> MSNLFRSLASSMRALSLAAPRATAVNTTKTVVSTHQTRCLSQGLLSRHICTPMCSHNRPVAVCQSAKNGLQSKQQSRGMKVHSAIKKRCEHCKVVRRKANKRQNGYLYIICPANPRHKQRQGYR;> MSTCQQVARPLVRCLRQTGPGAATCSTRSVAVAAVRPFSSTPMRKEEGATTTTTTSPVDSTTTPPPLPSATEAKATVADTVVGGPELGSRRRRAALATTGNLPFEQLPYQCFQDARKILQQDRAAKIAQIVKETEKIKLIEARDASEFEGGEAAKQTRIKSLRKYIEELKILADINDPEVKRRFEDGRGDMTKPVYRFMAERRWRSMDYKIIAQRISQFHVVPDLLPAFDPTMDVKLSFRGYQVSPGAILDSRVTEVAPTLRMQVFDKGERLLTVVVIDSDVPDVTHDNFKRRCHFLAANIPWDPSKTVLSLRSVGDRVEGDVGKPWLPPFAQKGSPYHRLNVFVLEQKPGAKIDGEALKKHLENRENFSLKGFREKFDLEPVGFNLFRSEWDEGTAEVMERHGIPGAEVEFKRQKFASLKPPRKARGWEAKRQKPKYKSLWKYVKRIA;> MVSATKKPVSAMSAKNSTRHRKVSHKVTKTIATAKSQVISNKAMKIRTKSWKDMPSPKRRRRINAMVDELRLQGNVKMPKPGKSTYKAGGGERVRLVKAASTLPTPPLTPPVLSKPTGSASQSKGDLKPKRPTPEKKRSVSKRDVERFFLSTQTSTRRRENTPIHAPIMSSTFTSLRGLATRLFAGGARPSPSSLLLPNKPATAALPTAIQHQQTASYASKGKSGPPAGMFSGQKAGSKKSKGPKQVDPRIINILRHFAVLSPKRIPPPLRFGRNRYLRHWTIHRAWLLFRRQQREQRERILMQQHQSMSNACEELRNTEGPGTRETGYLYRVAMLKNGVYGLKSIPIEYASRALVETPGRQAWNHEWKR;> MQPTRILQGLKYRKLRLTTKDVNKGFYKGNRTGSMGTHTSYGTYKIDYTKVRTYVCPDLTGFKLTPFVSKTIRPVHDQFPGDKLGPKNPATYLARWKSENGLD;> MTVKALTQISSAGRNGVGAFVLQCKKLDIHYSDWAGSSRGMNGFIKSLLPKFAAANPQIEFVVSPRPAKHPILMGHYINGRTKAICVRNMEPLEILKKAELLRDASGEKPQKFKKPVTSTNPSVRGVWSPYHGQGMAV;> MKRIATPSLTSRLLVAARSGVSPATAAIRSRSAISVRSQSTAALAQHDASHDLNNDRFPPLEPLPPAAESLPSPLPERALTSAKLAALHARLNLSPKIPLQTLARTLVDASADENPQFNNANLAFVGQTLINYHIAEWLLCKYPRLPQGILFSAMKAYAGPKPLLQIARSWGVDTAAVPGGEVDPGLLQFDALKPGVAITNFGYKRTELAYLEKFKWRRGMASRVVLDDDFGDVVRSDPKVAADLEKAMEEQDQDKTPDEEEAEMVANEQDQDVSYDRYGNPDTRAAAERAHAYFVRAVVGAIYAHCGREAAKAFVKAHIMSRTLDIAKLFEFKYPTRELAALCAREDFEPPVARLLSETGRQSRTPVFVVGIYSGSDKLGEGAASSLDHARFKAAMNALKAWYLYSPGENPRVPSDMLEEGAKPWTPAYIDMGEVISR;> MSASSRGAALLRSQQRSICLQCRNQTRVLAPAGVTSAPRRFYSAEASATATATATATTTTTLPPPHPPVTTSTGTHAATSTSSQIYRIKSGVILTRPPLLTRDLTPFEESFYFYQKRLNERLTAPFRKDFYFKKDTAADLDWRIKLKERHGVPAKDIGRYNPRGRMAWNDEVLVGSQTSSRKHMVEKLLADAEMRVSEDGEEIPAEDRVPVEKPMPRRTEADEKGDVKRLDRALDKTLYLVVKKKADKEGEEAKWMFPTGVVPTDEGLHETAARILAESAGVNMNTWIVGRVPVAHHVVRPVFGQKDGALLKKGEKIFFLKGRIMAGQADLTDNLHDLVDFKWLTQEELRSTLAEEYFHSVKGMFAER;> MFRSTFFGLSRAIVQPATPLTVRAAFQSRFYSAAAAASQPTTTATTTTPLQQQQQQQPTTQPTTPIQTQTGAAPTESTKPVAKPYLVGRAWTQRLPVYHLAKRGGNKKLTQIKKVQGDGQALRRDLAQFLGLEVKEVRVKVPTGHLEVDGHRREEIVKFLDGLGF;> MRRIPRIPSTASALCSSSSSVASTSAAPLRTLRAAADSSSICQSCSFSTQTSATRNRVWQNTVQTQRRCASTVTETTPEAPVAAAAAETATESTETVEQQRKRKGGFFETQRQVNLVLPGQPTRADAPEKIRDPNYEPATSGAGLQEIGGMSDWWSKPEHFRDGGKQFEYQGFAPQEKITDPRLLKVILRRALAEGLALKKFGANPKNPADMASIIGNGDHWQRTVSVEMCRGENGELSLKNESDLQKVWILMRNAAEKTYYQREWQEEINRLRSLGEKEQAKQLLEEGKKLGYRLKSEEGSLVKLTVDEAVELRKSWNNDWKEAIIRDPVVKFYAAKRIQKMTGHILSDGKLTSIQTVANFMDALVTPPKPKKLAEQIEQSSILPELPNVKVYPRRVTPVDKERMVGRWKVIQKELQKRELPVLGTGNHGKYVELKWLGSKQ;> MAALTPSRSVFASTCKTIAQQCSRRPVAVQQLAAVPVARQVSSSSAVQQEQDASGTSSSQQPRPRWSYTPERMKGPGFSLNLVKDPRRKQWMVNSDPAKLDAFYDAFLGQGGSRMLSEETKWLAVTHKSFDYGRRGYNTRLAFLGRQIIALETTRSILTSPVLNEPIVDKYGRTPYNHAALANIDKLIYTQPLDIMDKTKIARMGIDFGLLTVMRWKPRMPEDLESSGVVVVLNSTLFAIIGAISLEKGAAVAQRIVREKILKRLGA;> MLQPQFRPLLAGTASFAQTVLGRTVARCYATKAATQSASSTSTSNTSKDAKAKIVTPYVRDAGMMRTYKPHTPGIRHLKRPINDHLWKGRPYLPLTFPKKGQSKGGRNHSGRVTVRHRGGGHKRRIRMVDFERWIPGPHTVLRIEYDPGRSAHIALVKEEATGRKSYIVAADGMRAGDVVQSYRSGLPQDLLDSMGGVVDPGILAARTCWRGNCLPVSMIPVGTQIYCVGSRPDGKAVFCRSAGTYATIISKEEETREDGTKVMTGKFVNVRLQSGEIRRVSKDACATVGIASNIMHHYRQLGKAGRSRWLNIRPTVRGLAMNANDHPHGGGRGKSKGNRHPVSPWGTPAKGGYKTRRKSNVNKWVVTPRVRNMGVRRNKKTT;> MAPRLPARCWRQLSLVERSATHTTTTAAASSLLLAGRTTPTFSASSPSTVFPSLLPQITKRGVKYGWSTLPKRSRPTRFNQVTQGLPAPTSGPAAALKRREKTTPLRTGVLAVKKGMTVFMGRTGARIPCTVLQLDRVQVVANKTRAKNGYWAVQVGLGERRAENVGAPQLGYYEAKGIPPKQTLAEFKVRNQDGLLPVGVQLFPDWFHVGQVVDVRGITRGMGFAGGMKRHGFAGQEASHGNSLNHRTIGSVGGSQGSGSRVLPGKKMPGRMGAQQHTVQNLPILMVDNELGIVVVKGAVAGHKGAVVKVQDAVKKAPPPEEFVEATKQLLNERFPDAEEKLQAARKLHLELKEARRQGLIDSLIKNGLTEKADGNAAVEASA;> MAGKGLKSLNEAMNALSIASKSCRALPMRQSSILPCRRSMASVATPPAANITRSVSEPWQPITNVPVTVYSFPELEPRSLESYSARHLHLPLRRDILHLAVIYEGDSTRRGMASTKTRYEVHGSHKKMSPQKGTGNARRGTRQSPLMKGGGKTFGPKPRDFSTKLNKKVYDLAWRTALSYRYKRGELIVTEDGLDLPLPNDFLWLAGGGKLSRELEDGYVRKWVHEFMTSLNWGKEAGRTTFITGDKRPNLFTGFELAGAEGRALELWDVDVKDLLETGRIVIERSALKEMIEDHQSDLVTRVAVQGLRQKGPNLGEVLVRAPRY;> MASLRGVSRSARALQPFSAQFAVRRCASTQTGAGAAAATPKSNIPDLAELETRSALDAPIPSEEDKKEFRPWKRAADRKARLPSSRYQYHPPKYNRGPLHPIQSPPSSDPIARDFVPGPFNMPRLKETFRTVMASDLMTLAYIHTPPGTPKKEPTERLRAWEGDSPYFANRARRAPRGAPELPIRERDISFRNIPEIKEITVSTFVPLGLKNPDLLIVARAVLLAMTGTMPEMTRSKNNVVQWQLQANKPAGCKTTIYGNAAWEFMDRLIHLVLPRIKDWKGVPASTGDGSGNVQFGLNPEDVQLFPEVECNYDMYPAKMIPGCHIAIKTTATSDRQAKLLLQSLGVPFYSN;> MFAPSRRRVLEAVASSSSSPVVTLPGFLVPAFQQTAGAAARRNFSATTTRPSKLGRTPLSIPPGVEITIGEPFVKRDMTQWKQQPKRKITVQGPLGQLEMDIPDFIKIDHDAEARRATLSVANRDEKEQREMWGTTWAYLNRFIMGVSEGHTAVLRLVGIGYRATIDTRPEKEEYPGQQFVCLKLGFSHPVEMGVPKGMKASTPQPTRILLEGINREQVMTFAADIRRWRVPEPYKGKGIFVNGETIKLKQKKIK;> MSQTVGATRLAYSRVWHHISAVTPHPTLSTIKAPSEAITPPSLGRLASRIATILMGKHKPIWDPSTDCGDYVVVTNCAGLYTTGHKKWRKTYYRHNTRPGSLQAITMDALMEKHGGAEVLRKAVSGMLPKNRLRDKRLARLKAFEGDAHPYKENLVRFGGKVVGAPGWEEAVKAIREADMERL;> MIQLKTMLNCIDNSGAALVECAMVVGQKRHASIGDRIVVVVQKQRGADSAGMAASSAATKVKRGDIRHAVVVRTKQKVQRRDGSVVRFDDNACVLINKAGDPIGSRINGVVGQELRKKKWSKILSMAPMQA;> MPPRLPLAQAARCCQASLTARPSVPASSPTSSLISLFAALSVQTRSASILASLSDNRGAYHKRIRKGRGPSSGYGKTAGRGTKGQKAHGHVKPWFQGGQTPLIVSHGRKGFVNQFAADMSELNLEKLQEWIEAGRIDPTKPITPKEIIKSGIIGSSIKDGIKLLGRGKESFKIPVTITVSRASASAIEAIEAAGGKIVTRFYTKESLKRLVEGKSLHTDKPLPVGKEHVEEILAQARSLKKKYYRLPDPTSRWDIEYYRDPAHRGYLSHQLAPGESPSLYFKVPTGGEKVKVVRADKVKASKTGDVASEKLF;> MKHNASSALLSAFQGLRISSSATPFRAASLATSAVRRPIAPTPVSVASHVRLFSATAIQAGSWLEPNLNRKKKMMKGRPRVPTGGSTKGTTVVWGDYGLRMRDHHRRISAQQLKLAEDTIKQRLRGQKYRLYKRVACNVGVYVSGNEMRMGKGKGSFDHWATRVAVNQIIFEIRGQLHEQVIRDAFRLAGHKLPGLYEFVKKGDPPVVGITKLEDGLTVEDLKNPRKKLLMPEITQSAASTSSTAAPPS;> MAGAHVKYRHLSRSSAHRQALLRNLVTSLIKNETIHTTYPKAKEAQRLAEKLITLSKRDTETARRSAQGILYTPDQLLPKLFGEIRERYANRPGGYTRVLRTEPKDQYSQAPSAILELVDGPKDMRFAMTAATVARDREQKTESTDLTKKNMDKVTRFRKDGMRAFEDMVASLRDMKFTAGAINPKEWKKLDR;> MNVTASLSRRPLGCLKAGLCQSLIRGYATAVAASTTQSTGALPDHNFFRIADKHTKKTRTAFAVFTPPKSPTTLPPSSVVTKSKAFKIANSKLPPLMTKPPSDPMPLLTQQQIARMDPTGARTALFSKARHAARVGDVLMVTHRRGGEPFAGVCLAIRRSGIDTAILLRNHLGKVGVEMWYKIYNKNVAGIEIIKRRAKRARRAKLMYMRQPKHDMGSVEQYVFAWKKMRKVLSSKGLTGGVGGGGGKQKGQESKKKN;> MSRALLRSVLE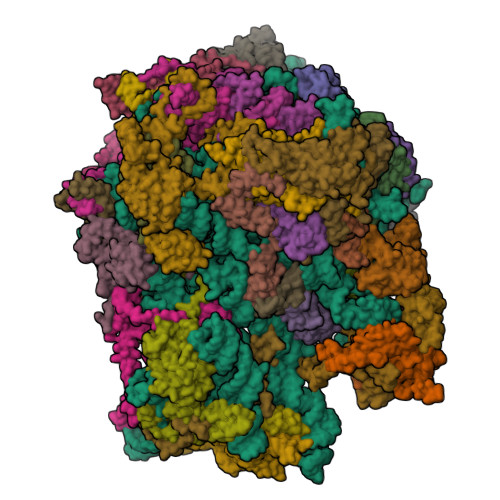LRTPVTRLPPSFLLPFRPAARFLHQTAQQVEPTSQSDAAAAAATLLKASPPKVTTATTPEAPAAVPTSTPFSQQPPISQQVKELLPVLAAQPGHYTTIHIHGKPYLVTEGDTVKLPFKMPGVAPGDVLRLNRASVIGSRDLTLQGAPYVDERLFECRAIVMGTESEPMRVMIKKKRRCRKKKHVFSKHKYTVLRINQLKINDVSSL;> MSLNVPSRRLLKSAPSSANALVPALQSLSINTRSIHTTPSQQWSLFGWGKQKVEERNKVKEELKQSELARTRKPTQEEIFERVRGRLEGDSIFADTTPSSQLAAEQDKHKDWATASAEKKLAAAHAKDQTPTGISLKKDHLVRVVDPDPRSRVRWERKMVIRKLQRGTDPWSVEPKAERIARTERKLVYKTGYLPTSVKKLVHLSRQIRGKTVSEALVQMQFSKKKMAKEVKTELLRAEAKAIVTRGMGLGKAAAAAAQKETGAEPVKIQTKDGKHLEIRDPTRIYVAETFVNKGFTRGVELDYRARGRVFKMNKPTTTMTVVLKEEKTRIREHQERVAKKLRQGPWVHLPDRPVTSQRQFYSW;> MASVAKTGAEALRNAPFRVGKKQIFLPNHVITFVRPLPKQPPNLATFIVPLEFNKLDLRDYLYHVYNVEVTGVRSFVNQRMHEQRHGDVGNWRRPKSQKMMIAELAKPFVWPKPPAEDAREAFDYAMWKKQKTAQEQDTKFQGIRAQGEVVPPSQFEVTKDRKAIKARQSKFLSGEETWAPGKVNAFLNSKIVPEEEGWSEVEENLPLDESAESAAEESSSKGSETRQ;> MDKLLRRVRMAEGMVARRAQRKNALLKRITERKQNKKNGEAFTEAIQQRKAAVEARNEDWMLGPLAPRRELDEITLSNGNFFGSLSPTRALLESEVSEEERKARVAWCGSPKFLCIAPGDRVVVIEGHHKDLIGTIEKLNTRNMTVEIQSEKLKTNTTVPQFMQNDADKPVTQIYARLPISSVRLVHPLKDPQTGEYRDVIIRELRPRNIVHDRPTRTRSMRRFVPGENIIIPWPKQEPIKREDQPADTLRIDVDEKTFVPTLFRPPAPQQVLDELRNKYSIFRTRHTPEYIAKKEQEEQEKEAKKSAAKAMLTPVQEYNRKQRELRRARGQPALTEEMLAKIGEVVARNKLGHHQAPKVKEETVAQIEKAVEQLSLGGGQEDAATTTSPEQPKVV;> MHLAQLRQPLTRAAANSCHSVCRLPTTHSSVSATAILSEQFAHLRIGPSSSNVAVEGRRYASVKAQGAYRLKPKRTIPKKLGAKKTGDQYVIPGNIIYKQRGTLWHPGENTIMGRDHTIHAAVAGYVKYYRDPQLHPDRQYIGVVFNRNDKLPYPKDAPRKRKLGLVAVPRKVEEVEKPTMSASGLPLFVTRHETIEIPPPAVTTPAAAGKAVKGQGARVSASGAAAVPASSSTISASASSNSNNGGSSVIAELIKEKLAARAEYNARQSALRKLQQQKMLARRGTRVLRLMNNYSYRETNWEIGRLIGDPGSVPGTEKVGSRKAKFRARRRRRNTFLLGIKERKLAKADRREEYRRRVREKREQRLVQRKEFLAKQREAKKAREGGAAAEKSEKKEVKAEKPAAAAPKVEKPKAPEAAKKESKPKVEEKKAAAAEPKKDSKTEKKD;> MSSFLVRPFCLRATTTTTTTTTTTALVQQQLRALTTTTALTYHQPRVPSSAIPIPNVSGRVPLPDSTPVPEDFKIEIPSYPYGPRRVYHQSNTGLYGSALIRFGNNVSKRNEIKTRRKWRPNVQQKRLWSKSLGVFVRTRVTTRVLRTIDKVGGLDEYLLGHKAARVKELGPWGWMLRWRIMQTPEIRERFAKEREALGLPPRREEDEEKSLEEQLREFQVAGIQFAEGKAPKTKGQLKEEADRLIKKSETEEFGLGQEEDLFMKEEPKPTKMA;> MASPAALRPSMGAIMQTCRSAATAPKVAVAVPVRALSTSAALLKRHKYPTARVTRDNSKQRGESALRKSGTRWKLSVSDEPLPEPVPREELPPIQVDENHGLWDFFYDRETVAMAPLEHTKHGRAWTVSELRKKSWDDLHRLWWVCVKERNRIATANWERTKSELGFGLAEANERDRNVKQTMRGIKHVLTERFYAWEDAVKLAEQDPEIDLSNPENPYTPSTFLEAEETAEGAEASETQSTTTEIDPTTIPSSKSQAEAPRV;> MSFFRITLHRSAIGLPKRTHGVLAALGLRRRNQTVFHPVEPQFAGMLMKVKELVRVEEVPHRLTKRELKDERKPDAGFVVEKQVRRFIPGVGVQDEVDFSKVVEELKAQKVENVEGVEKMVVEGGAVVRDGKRAGDLGVRTRSDWEVIGKMKSVLPKVKAL;> MSSKLPTTLLRRPSALPSTTTYTAYSASRPTPPSCTAHGAQGQQIRNATFVPRHRRPYQFTQLVQLSDGSTFTVRTTMPTALYKSAKDSRNHLLWQPSDKSLKNVELDEAGKLAAFRERYGRGWDLDAKMTPEEEAAAAAALAAGGGAGVPGGKAAKKAAEEALLAKKKKEEEEAAKKAAEAEEADPFDSLTDLISGYATENMNPGLNFKETRHYGKKK;> MAAMTAAAAAPAMRLFNPSTFFQTLRTQRFGVPALNFAVPAAAISLLPSIPSLLEDIWEGILRAVPKKKTSHMKKRHRQMAGKALKDVTHLNRCPACGNLKRMHHLCSTCLGKLKGFMDRNGGSNAKAY;> MAKKAKSRIINVRLISMAMTGYFYTFTRPRTSLPMSMLKYDPIVRRKVLFLEQKRKGRS;> MSRIFSSALQAVFKPSAFLPKTATRSFSILPSLRPATLSSTPSTIFRAPNAITAPSASPSATTGIDGEVLDLLSASSLISSHPALSGLGSQIRCGPRPTMSGATRLVQKRRHGFLSRVKTKNGQKTLKRRLAKGRLRLSA;> MEASLSLFRPVATCCRRVALSSSSSSSQKAAAVAGISVRYQSTANRTKRMLNIPPHESFLNVPVEGDRIIFNPPSSEASVYHTPFKFLPRSDPRRRANIYKLFKPPQAPITTPESSSTDAAAADQHGDLPPVLYNPTKSYNVTPEQVEEIRELRAKDPKKYSVTYLSNKYNCTKVFIMMCTQAPREHQEQHKLARARTAENWGPRRAAAKLDARRRKEMLHRGEI;> AATVKQHVQLALSLPPRLRTFLARYPPASILPAGADPETHKTPYQEESPNPFMPTKHPITGKWHNPKYSLRRQAELVKLAQEHGVEELLPFTRKLNEEKLRKRVELGLRVKGTGVGEKVKGHKHERTLVAKMEKRREAMLAMPDLIREWKKVGKRNWTKFPK;> MFGAFRFTNPLSGGLLWKIPWRMSKFQKLRQRRRLRAVDNVVATIENALAKKGETVKAVERWRAEMPTEAEMLPKDKYTIFDRKEKRYRKGIHKLPKWTRVSQRVNPPGY;> MNSVTTSTIGRLAFGVSRLSAVTNVAGAVRHASTHPTTAIPKPTTAVLKTSPLAEETAVELKSPSRLQLKSEPGNKGNPKGHGDRIWAFHHIEQGQVIYSTKPVISHQHLIRQQPFTGKNLVPRKIRKDYWRPLAMIELAGKDQGAVGRSVYQKLREFKKRHELDWANEAEEGRKLMHKSKRERGQELNDQKPNSVADMAAVLAGAGKGNLMWQVSRLGSSSELVGEIKKASGAVEKGAVVDVKRQLRRATVYWTNEQDKFHAREWSDNVSHEVGIPGEAEKKRMPIRMSSE;> MSLRLSRPAVRGLGSAIKSSRISSRSAALLVPSTSTSAFSTASPQRAAAAGHLRLPDDYVPPTQPPSARPVDTRKSQLLRTYTSMLRSTPLMLIFQHNNLTAIEWAAIRRELSLALSNVPVPEGAPDITSKIHLQVVRTRIFDVALKTVEFFDPSTVEPTTATTATGTKVPATYNHDLSKHAWKAVKEATKNTEAVEKTVYGQLAPLLVGPVAILTLPSVSPAHLGAALSVLAPSPPAFPAPSRKKNPGYYDLTCQSGLQKLLLVGGRIEGKAFDYDGIKWVGGIENGIEGLRAQLVHMLQSAGMGLTSVLEGAGKSLWLTMESRRSVLEEEQNPKKEGEGEEEKKE;> MSKAAKGGAGGVEQVVKLIVGAGQASPSPPVGPALGSKGIKSMDFCKEFNARTAHINTGTPMPVRVTVRPDRSFHFDVRTPHTSWLLLNAAEAPIGKGGKRKGASNPGKEVVGTVSLKHVYEIAKIKQSELRLSGLPLEGLCRAVIYQARSIGINVIP;> MLTRFITDVSTRFNPFSAKAKAARLFLSFLPPNARSNGMNITTQLLPRNSTETPLLYVKFKDGKEMNLDVENMGIKSIVEEVDRHSRILQKQADLNDG;> MICRTCLRRASGFARPAAAAATRPMVAASSRAAFSTTFSVCTPPAATPAAAAPATSTAEAGLAPVPGAATTEQAKAAISSCPAGTKLNGLNYFKNKADPVALPDEEYPEWLWRCLEVQKKTDDAADADAGDEFSKSKKQRRLAMKRARAQEAKILASGDLEALAPKIPLQKQSVNLPGAVNGGVQDAVLADEKREELRKAMRKERKAKIKESNYLKAM;> MSATPAVLRASACSACRFSALRLFVSSFASPRAPLPVARTRVLSPTAPYSTFRPSPRLLASPSSEEHAEPAAQEQPNKTEDAQAEASTEANNEGGADVPWYLQVDAPTHPTLVHEPPPLPDIPEGSPKLMEPLVKFVSDELGMDDLKLLDLREIDPPPALGPEVLMLFGTARSERHLHVSADRLVRWLRNRGVTAKADGLLGRNELKTKLRRKARKAKLLGTTGLPSGADDGITTGWICVNLGTLGWSDMEMEFKDEKGVTSGFGVPQSGTTLVVQLMTETRREELALEKLWSGILRRSLERQDKIAGKLPEASFTTSPDTVSGQSFSPSPIRSSGRNRKRPDRLYFSTSARQHAAAVDVSQTDLATAMAGWEYSNASPSTIDNLLAQDTDSKVQLLIQMQEYLSSLPRDQALSAVSLCEDGSPSTFMRLFNRAIENLPSAQAWEARLWVEKAARALQHPDHDLARLGDLIQEMKLSGAANVSREKFVDLLRMIFAIPETTDAGVRQQASLSMDVIDMLFSRGEKVIEYDVVVAVIESLLQTRARPPEARRLLSQFEDLLSEAQMDCPTEDEIIRLLDVYANHRAWDKFWNVWRVFPRHCERRTERMYTKVYERIAAEDHQGMATDALRWCVEEMWHEQPPVRVTAAMLKALEACIRIADPEAESLAKDIDDRISDAQYMDREFVRLWLTLHGSAAWGA>[8x]MSVSAFNRRWAAVILEALTRHGVRHICIAPGSRSTPLTLAAAENSAFIHHTHFDERGLGHLALGLAKVSKQPVAVIVTSGTAVANLYPALIEAGLTGEKLILLTADRPPELIDCGANQAIRQPGMFASHPTHSISLPRPTQDIPARWLVSTIDHALGTLHAGGVHINCPFAEPLYGEMDDTGLSWQQRLGDWWQDDKPWLREAPRLESEKQRDWFFWRQKRGVVVAGRMSAEEGKKVALWAQTLGWPLIGDVLSQTGQPLPCADLWLGNAKATSELQQAQIVVQLGSSLTGKRLLQWQASCEPEEYWIVDDIEGRLDPAHHRGRRLIANIADWLELHPAEKRQPWCVEIPRLAEQAMQAVIARRDAFGEAQLAHRICDYLPEQGQLFVGNSLVVRLIDALSQLPAGYPVYSNAGASGIDGLLSTAAGVQRASGKPTLAIVGDLSALYD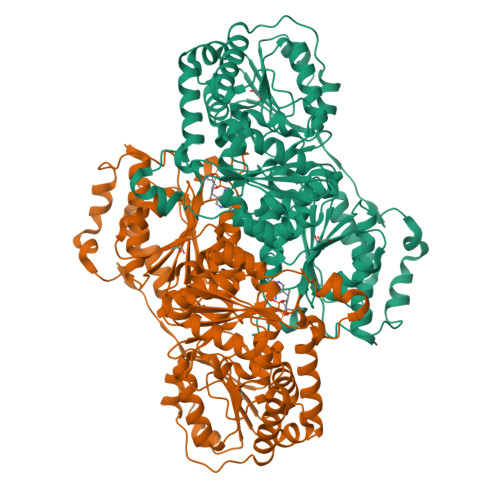LNALALLRQVSAPLVLIVVNNNGGQIFSLLPTPQSERERFYLMPQNVHFEHAAAMFELKYHRPQNWQELETAFADAWRTPTTTVIEMVVNDTDGAQTLQQLLAQVSHL> MTTSHGLIESQLSYYRARASEYDATFVPYMDSAAPAALERLRAGNIRGDVLELASGTGYWTRHLSGLADRVTALDGSAEMIAEAGRHGLDNVEFRQQDLFDWTPDRQWDAVFFAHW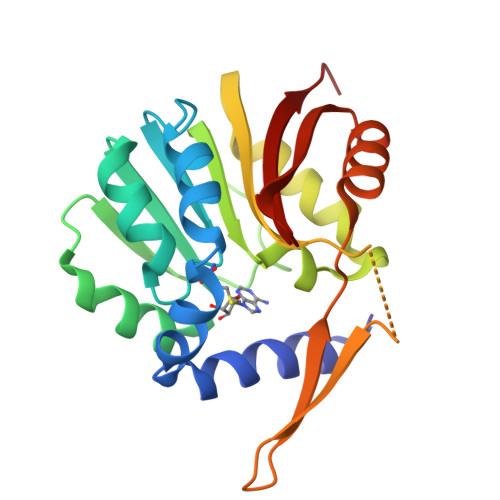LAHVPDDRFEAFWESVRSAVAPGGVVEFVDVTDHERRLEQQDDSEPEVAVRRTLQDGRSFRIVKVFRSPAELTERLTALGWSCSVDEVHPGFLYATCRPGPR One widely occurring ribonuclease with such multi-functional versatility is polynucleotide phosphorylase, a phosphorolytic exoribonuclease (PNPase; polyribonucleotide nucleotidyltransferase; EC 2.7.7.8).5,6 PNPase processively cleaves single-stranded RNA substrates in the 3′-to-5′ direction using inorganic phosphate to attack the phosphoester linkage at the 3′ terminus and liberate nucleoside diphosphate. E. coli PNPase core forms a homotrimer with a ring-like architecture that encloses a large central channel. The two RNase PH-like domains within each protomer are spatially related by a pseudo-dyad axis, so that the PNPase trimer has approximate dihedral symmetry D3. In the current study, we solved several crystal structures of E. coli PNPase core bound to its cognate RNase E micro-domain, including a complex with O2′-methyl-modified RNA bound and another with manganese in the active site.

We find that Mn2+can substitute for Mg2+to support catalysis (S.N. et al., unpublished results), and since Mn2+can be more readily identified in difference maps and anomalous Fourier syntheses, we prepared RNA-free co-crystals of the PNPase core in the presence of 20 mM manganese acetate. In this crystal form, a single protomer occupies the asymmetric unit, and the map revealed clear density for Mn2+at the active site. Mn2+is coordinated by the conserved residues D486, D492 and K494 (inset), and it is likely that magnesium will bind in a similar manner. The metal-coordinating residues D486 and D492 may act in conjunction with the bound metal to support general acid/base catalysis. The RNase E micro-domain is also well resolved in the rhombohedral crystal form with Mn2+ but was poorly resolved in the second rhombohedral form grown in the absence of the metal. Guided by this overlay, a model for the transition state of an RNA substrate under attack by PNPase was prepared. Lastly, we docked the chimeric RNA structure from the P. abyssi exosome structures onto the corresponding position in our PNPase core-manganese structure. The overlay shows that the metal is in a good position to support the proposed transition state. The metal is well orientated to interact with the carboxylates of D486 and D492, and the pro-chiral, non-esterified oxygens that are in the axial position of the bi-pyrimidal transition state. In the RNA-free structure, the metal is coordinated by water molecules at the positions that correspond to the phosphate oxygens in the transition state.

> MLNPIVRKFQYGQHTVTLETGMMARQATAAVMVSMDDTAVFVTVVGQKKAKPGQDFFPLTVNYQERTYAAGRIPGSFFRREGRPSEGETLIARLIDRPIRPLFPEGFVNEVQVIATVVSVNPQVNPDIVAMIGASAALSLSGIPFNGPIGAARVGYINDQYVLNPTQDELKESKLDLVVAGTEAAVLMVESEAELLSEDQMLGAVVFGHEQQQVVIQNINELVKEAGKPRWDWQPEPVNEALNARVAALAEARLSDAYRITDKQERYAQVDVIKSETIATLLAEDETLDENELGEILHAIEKNVVRSRVLAGEPRIDGREKDMIRGLDVRTGVLPRTHGSALFTRGETQALVTATLGTARDAQVLDELMGERTDTFLFHYNFPPYSVGETGMVGSPKRREIGHGRLAKRGVLAVMPDMDKFPYTVRVVSEITESNGSSSMASVCGASLALMDAGVPIKAAVAGIAMGLVKEGDNYVVLSDILGDEDHLGDMDFKVAGSRDGISALQMDIKIEGITKEIMQVALNQAKGARLHILGVMEQAINAPRGDIS;> EAPRHSDWQRPTFAFEGKGAAGGHTATHHASAAPARPQPVE>SNAQITFVSQGGAYQAAQTVAILDPSAKKLGITINQDSIPDAWPAIKTQVGSGKPIWDVVDTPTGYCLRGGEQGLIEKLDFSKIPNAAAMPEAYRSPYSVSYEFYSSVLAYSQKTFPKDAPNSWVDFWDVKKFPGRRALRNHPIATLEAALMADGVAPDKLYPL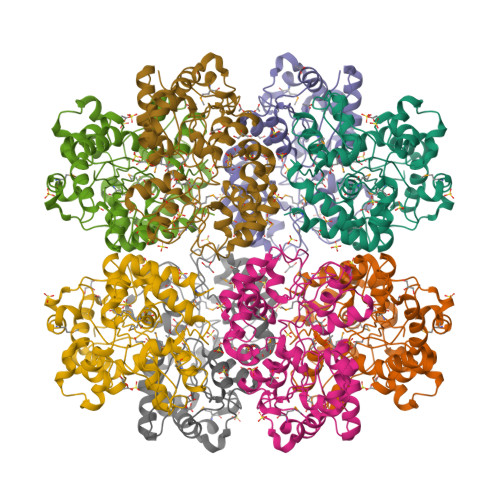DVDRAFKKLEEIKPHITVWWTSGAQSAQLLNDGEVDMEMAWNGRVSAVAKEGAKVSFTYNQGILQSTSLCILKGAPNLETAVKFLNEAVDPVHQANLPLHIDYGPGNPKAFETNVIKPERAAQLPSEPANAAKQALMSYAWWSSPAGEAAEKRWASFMQK[4x]> GCACCTGT;> ACACCG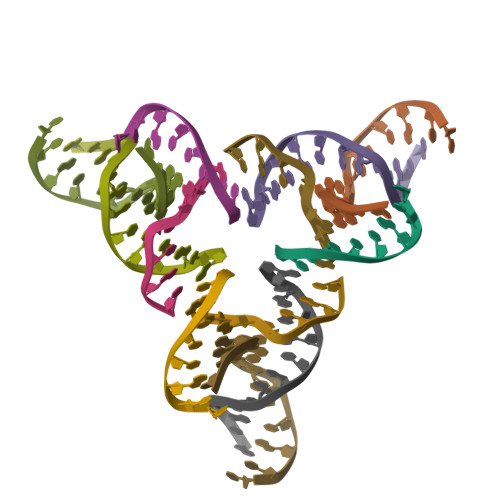T;> CTGCTACTGTGGTG;> ACGGACAGTAGCA> MSHHHHHHHSKRHIPVVTDIYSIEDHRLEDTTHLQYAPNAIKTEGKGSGSGPAVCKKVTEHEKCTTSIMDKLTAFFGVMPRGTTPRAPVRFPTSLLKIRRGLETGWAYTHQGGISSVDHVTCGKDLLVCDTMGRTRVVCQSNNKMTDESEYGVKTDSGCPEGARCYVFNPEAVNISGTKGAMVHLQKTGGEFTCVTASGTPAFFDLKNLKGWAGLPIFEASSGRVVGRV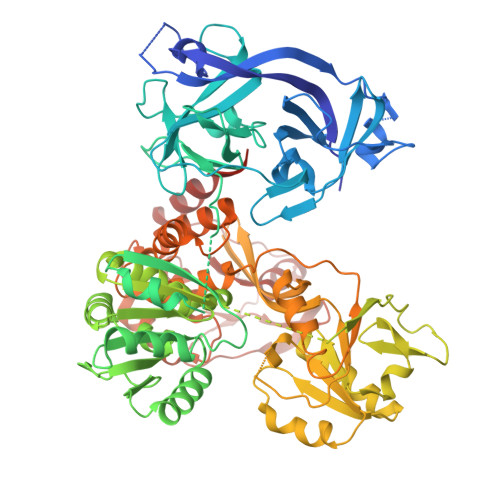KVGKNEDSKPTKLMSGIQTVSKSTTDLTEMVKKITTMNRGEFRQITLATGAGKTTELPRSVIEEIGRHKRVLVLIPLRAAAESVYQYMRQKHPSIAFNLRIGEMKEGDMATGITYASYGYFCQMPQPKLRAAMVEYSFIFLDEYHCATPEQLAIMGKIHRFSENLRVVAMTATPAGTVTTTGQKHPIEEFIAPEVMKGEDLGSEYLDIAGLKIPVEEMKSNMLVFVPTRNMAVETAKKLKAKGYNSGYYYSGEDPSNLRVVTSQSPYVVVATNAIESGVTLPDLDVVVDTGLKCEKRIRLSSKMPFIVTGLKRMAVTIGEQAQRRGRVGRVKPGRYYRSQETPVGSKDYHYDLLQAQRYGIEDGINITKSFREMNYDWSLYEEDSLMITQLEILNNLLISEELPMAVKNIMARTDHPEPIQLAYNSYETQVPVLFPKIRNGEVTDSYDNYTFLNARKLGDDVPPYVYATEDEDLAVELLGLDWPDPGNQGTVEAGRALKQVVGL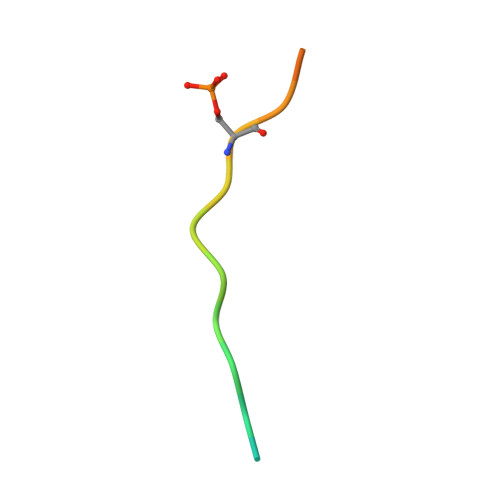> STLTEEFELLISNSEDDWE> SDVAFRGNLLDRPCHVSGDSLNKHVVFKTRASRDFWYPPGRSPTESFVIRLENCHATAVGKIVTLTFKGTEEAALPGHLKVTGVNAGRLGIALLDTDGSSLLKPGTSHNKGQGEKVTGNSLELPFGAYVVATPEALRTKSVVPGDYEAT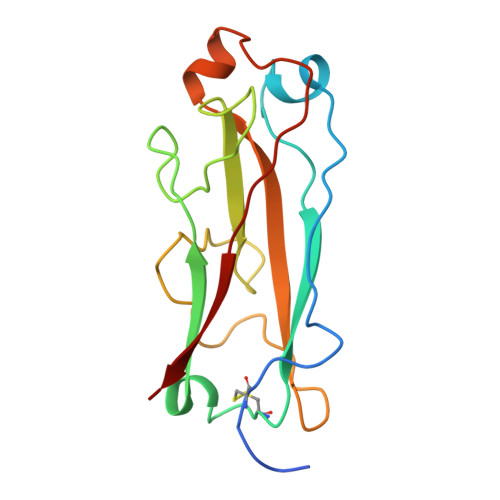ATFELTYR Here, we demonstrate that DC3000 produces IAA and identify an indole-3-acetaldehyde dehydrogenase, AldA, that catalyzes the NAD-dependent formation of IAA from indole-3-acetaldehyde (IAAld). The AldA monomer adopts a canonical aldehyde dehydrogenase fold, which contains an NAD+-binding domain with a Rossmann-fold motif of a central β-sheet (β10-β9-β8-β11-β12) surrounded by α-helices, a mixed α/β domain with the catalytic cysteine residue (Cys302), and an oligomerization domain with a protruding β-sheet (β6-β7-β23). In each structure, two AldA monomers were in the asymmetric unit and packed to form a dimer, which then form a tetramer by crystallographic symmetry. Overall, the biochemical and structural data presented here indicate that in P. syringae strain DC3000 AldA functions as an IAAld dehydrogenase in IAA biosynthesis.

The x-ray crystal structures of AldA in the apoenzyme, NAD+ complex, and NAD+•IAA complex forms were determined. Comparison of the AldA crystal structures suggests that ligand binding results in structural changes that order the active site. The α11-β14 loop (residues 297–305), which contains Cys302, is disordered in the apoenzyme structure and has average temperature factors ~1.8-fold higher than surrounding residues. Likewise, a ~50 amino acid region of the catalytic domain (residues 348–397; α13-β15-β16-α15-β17-β19) is disordered in the apoenzyme structure and displays elevated B-factors in ligand bound structures. In the reaction sequence catalyzed by AldA, substrate binding leads to conformational changes that order the active site for catalysis.

>MTTLTRADWEQRAQNLKIEGRAFIQGEYTAAASGETFDCISPVDGRLLAKVASCDAADAQRAVESARSAFDSGAWSRLAPAKRKATMIRFAGLLEQNAEELALLETLDMGKPISDSLGVDIPGGARALSWSGEAIDKLYDEVAATPHDQLGLVTREPVGVVAAIVPWNFPLMMACWKLGPALSTGNSVVLKPSEKSPLTAIRIAQLAIEAGIPAGVLNVLPGYGHTVGKALALHMDVDTVVFTGSTKIAKQLMIYAGESNMKRVWLEAGGKSPNIVFADAPDLQAAADSAASAIAFNQGEVCTAGSRLLVERSIKDRFLPMVIEALGTWKPGNPLDPATNVGALVDTQQMNTVLSYIAAGHTDGARLVAGGKQILQETGGTYVEPTIFDGVNNAMRIAQEEIFGPVLSVLTFDTAEEAIQIANDTPYGLAAAVWTANLSKAHLTARALRAGSVWVNQYDGGDMTAPFGGFKQSGNGRDKSLHAFDKYTELKSTWIKL[2x]> MAPRANTKIIVVGGGGTMGSSTALHLLRAGYTPSNITVLDTYPIPSAQSAGYDLNKIF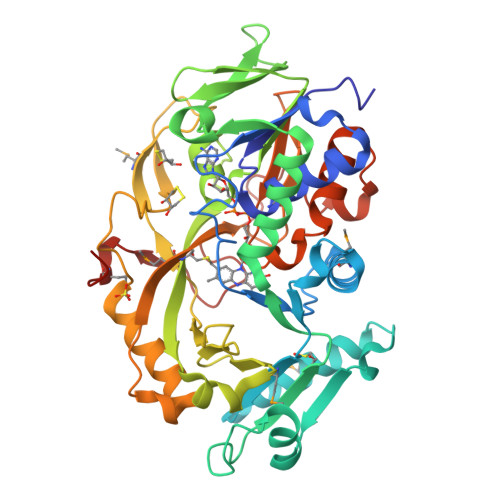GIRLRNKPDLQLYLEALDMWKNDPLFKPFFHNVGQMDVSSTEEGIKKLRMRYQSLLDAGIGLEKTNFLLESEDEILAKAPHFTREQIKGWKGLFCGDGGWLAAAKAINAIGQFLKEQGVKFGFGEAGTFKKPLFADADEKTCIGVETVDGTKYYADKVVLAAGAWSSTLVDLEEQCVSKAWVFAHIQLTPAEAAAYKNTPVIYDGDYGFFIEPDENGIIKVCDEFPGFTHFKMHQPYGSPVPKLISVPRSHAKHPTDTYPHASEVTIKKAINRFLPRFNDKELFNRAMCWCTDTADANLLVCEHPRWKGFYLATGDSGHSFKLLPNIGKHVVELLEGRLESVFKDAWRWRPGSGDALKSRRAAPAKDLADMPGWRNEAKM> SINGGIRAATSQEINELTYYTTLSANSYC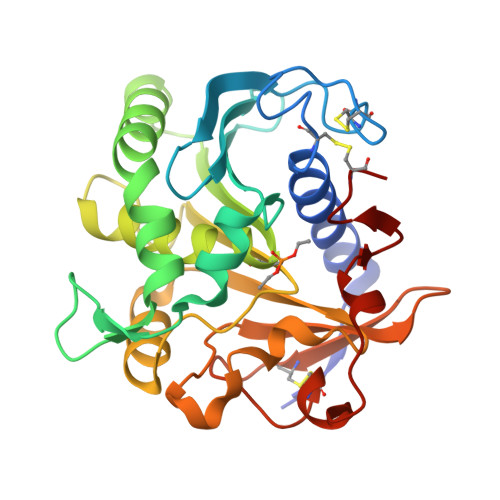RTVIPGATWDCIHCDATEDLKIIKTWSTLIYDTNAMVARGDSEKTIYIVFRGSSSIRNWIADLTFVPVSYPPVSGTKVHKGFLDSYGEVQNELVATVLDQFKQYPSYKVAVTGHSLGGATALLCALDLYQREEGLSSSNLFLYTQGQPRVGNPAFANYVVSTGIPYRRTVNERDIVPHLPPAAFGFLHAGSEYWITDNSPETVQVCTSDLETSDCSNSIVPFTSVLDHLSYFGINTGLCT> GNYN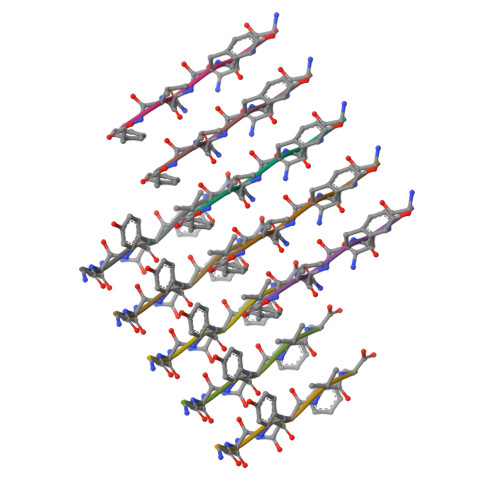VF> GPLGSEVIQALIFKDDGSL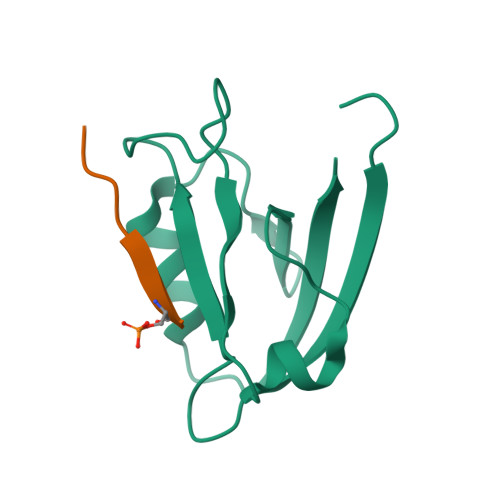GLSISGGVGSSSFKSGDDGIFVSKIAKGGPCDNEGTLKIGDKILSVNEISFTGITHEKAVEILKNQDSKYMVVVERS;> NPNPETSV>GAMENIAPVARFELKVEGLSVMSQNTSSDSDGNIVSYLWDFGNGQTST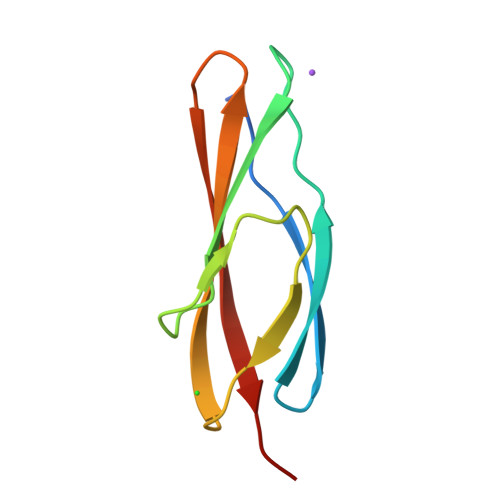EAAPTWSYTKAGSYSVTLTVTDDKGDSDTHQQTIKVDTPN[2x]> LH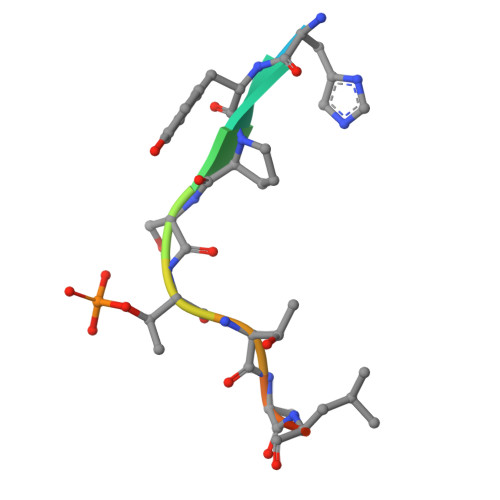YPSTTALQE~{N}-[5-(azepan-1-ylsulfonyl)-2-methoxy-phenyl]-2-quinolin-4-yl-ethanamide | C24 H27 N3 O4 S | 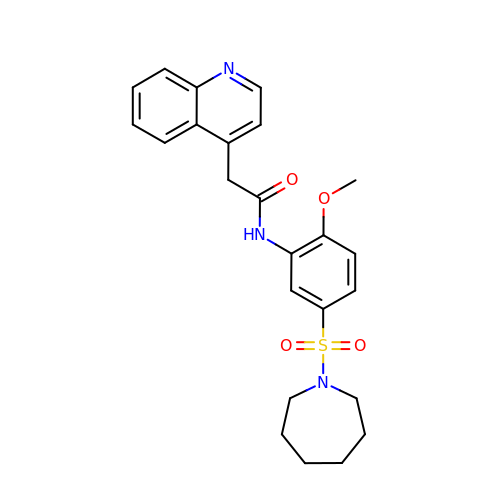NMFIWQRACOVPFY-UHFFFAOYSA-N> RYNVTA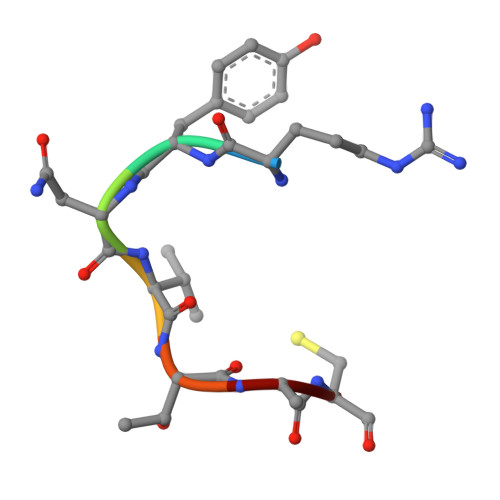C> TNE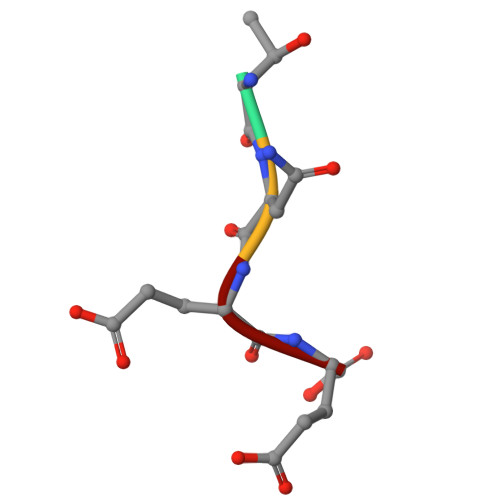E>[2x]MGNVLVVIEQRENVIQTVSLELLGKATEIAKDYDTKVSALLLGSKVEGLIDTLAHYGADEVIVVDDEALAVYTTEPYTKAAYEAIKAADPIVVLFGATSIGRDLAPRVSARIHTGLTADCTGLAVAEDTKLLLMTRPAFGGNIMATIVCKDFRPQMSTVRPGVMKKNEPDETKEAVINRFKVEFNDADKLVQVVQVIKEAKKQVKIEDAKILVSAGRGMGGKENLDILYELAEIIGGEVSGSRATIDAGWLDKARQVGQTGKTVRPDLYIACGISGAIQHIAGMEDAEFIVAINKNPEAPIFKYADVGIVGDVHKVLPELISQLSVAKEKG;>MNIVVCI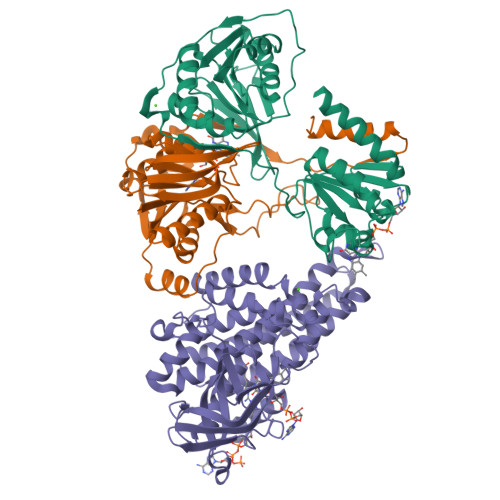KQVPDTTEVKLDPNTGTLIRDGVPSIINPDDKAGLEEAIKLKEEMGAHVTVITMGPPQADMALKEALAMGADRGILLTDRAFAGADTWATSSALAGALKNIDFDIIIAGRQAIDGDTAQVGPQIAEHLNLPSITYAEEIKTEGEYVLVKRQFEDCCHDLKVKMPCLITTLKDMNTPRYMKVGRIYDAFENDVVETWTVKDIEVDPSNLGLKGSPTSVFKSFTKSVKPAGTIYNEDAKTSAGIIIDKLKEKYII[2x];>[2x]MDLNSKKYQMLKELYVSFAENEVKPLATELDEEERFPYETVEKMAKAGMMGIPYPKEYGGEGGDTVGYIMAVEELSRVCGTTGVILSAHTSLGSWPIYQYGNEEQKQKFLRPLASGEKLGAFGLTEPNAGTDASGQQTTAVLDGDEYILNGSKIFITNAIAGDIYVVMAMTDKSKGNKGISAFIVEKGTPGFSFGVKEKKMGIRGSATSELIFEDCRIPKENLLGKEGQGFKIAMSTLDGGRIGIAAQALGLAQGALDETVKYVKERVQFGRPLSKFQNTQFQLADMEVKVQAARHLVYQAAINKDLGKPYGVEAAMAKLFAAETAMEVTTKAVQLHGGYGYTRDYPVERMMRDAKITEIYEGTSEVQRMVISGKLLK>HFLCGVVEGFYGRPWVMEQRKELFRRLQKWELNTYLYAPKDDYKHRMFWREMYSVEEAEQLMTLISAAREYEIEFIYAISPGLDITFSNPKEVSTLKRKLDQVSQFGCRSFALLFDDIDHNMCAADKEVFSSFAHAQVSITNEIYQYLGEPETFLFCPTEYCGTFCYPNVSQSPYLRTVGEKLLPGIEVLWTGPKVVSKEIPVESIEEVSKIIKRAPVIWDNIHANDYDQKRLFLGPYKGRSTELIPRLKGVLTNPNCEFEANYVAIHTLATWYKSNMNGVRKDVVMTDSEDSTVSIQIKLENEGSDEDIETDVLYSPQMALKLALT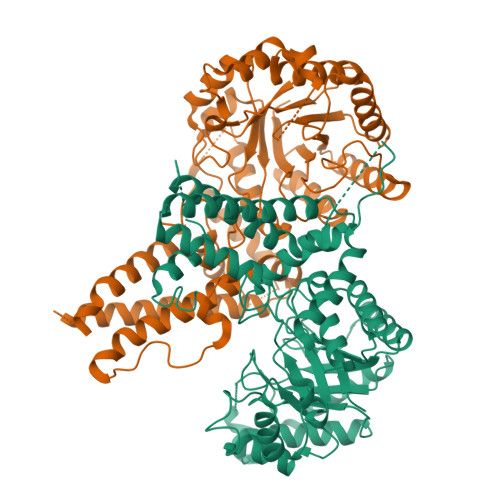EWLQEFGVPHQYSSRGGGGSGGGGSVTLEDLQLLADLFYLPYEHGPKGAQMLREFQWLRANSSVVSVNCKGKDSEKIEEWRSRAAKFEEMCGLVMGMFTRLSNCANRTILYDMYSYVWDIKSIMSMVKSFVQWLGCRSHSSAQFLIGDQEPWAFRGGLAGEFQRLLPIDGANDLFFQ[2x]>MRVGIPTETKNNEFRVAITPAGVAELTRRGHEVLIQAGAGEGSAITD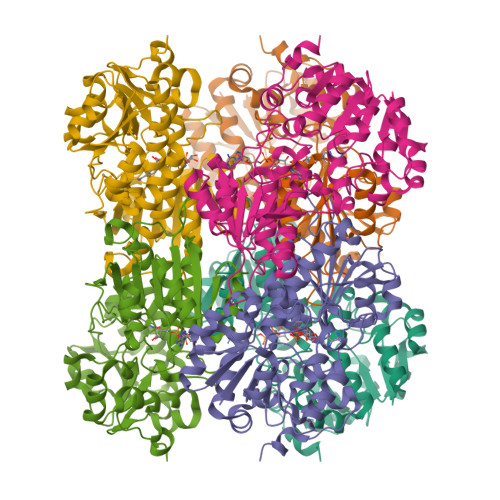ADFKAAGAQLVGTADQVWADADLLLKVKEPIAAEYGRLRHGQILFTFLHLAASRACTDALLDSGTTSIAYETVQTADGALPLLAPMSEVAGRLAAQVGAYHLMRTQGGRGVLMGGVPGVEPADVVVIGAGTAGYNAARIANGMGATVTVLDINIDKLRQLDAEFCGRIHTRYSSAYELEGAVKRADLVIGAVLVPGAKAPKLVSNSLVAHMKPGAVLVDIAINQGGCFEGSRPTTYDHPTFAVHDTLFYCVANMPASVPKTSTYALTNATMPYVLELADHGWRAACRSNPALAKGLSTHEGALLSERVATDLGVPFTEPASVLAHHHHHH[2x]> MGSSHHHHHHSQDPNSTTTAPPVELWTRDLGSCLHGTLATALIRDGHDPVTVLGAPWEFRRRPGAWSSEEYFFFAEPDSLAGRLALYHPFESTWHRSDGDGVDDLREALAAGVL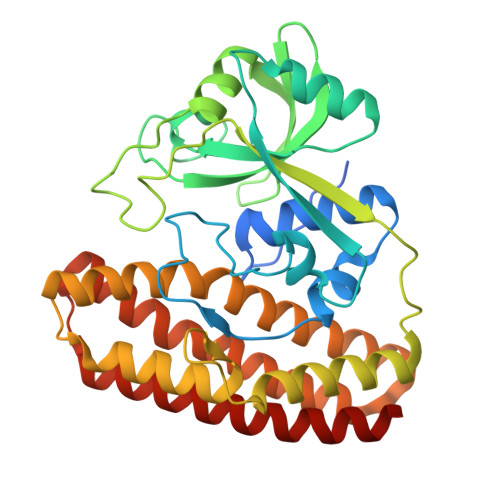PIAAVDNFHLPFRPAFHDVHAAHLLVVYRITETEVYVSDAQPPAFQGAIPLADFLASWGSLNPPDDADVFFSASPSGRRWLRTRMTGPVPEPDRHWVGRVIRENVARYRQEPPADTQTGLPGLRRYLDELCALTPGTNAASEALSELYVISWNIQAQSGLHAEFLRAHSVKWRIPELAEAAAGVDAVAHGWTGVRMTGAHSRVWQRHRPAELRGHATALVRRLEAALDLLELAADAVS> MDIVDGDQCESNPCLNGGSCKDDINSYECWCPFGFEGKNCELLEHH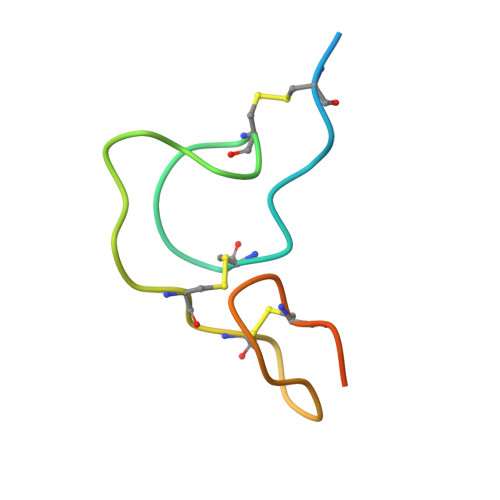HHHH>SNAESKIKDCPWYDRGFCKHGPLCRHRHTRRVICVNYLVGFCPEGPSCKFMHPRFELPMGTTEQ[4x];>SNAGSINGVPLLEVDLDSFEDKPWRKPGADLSDYFNYGF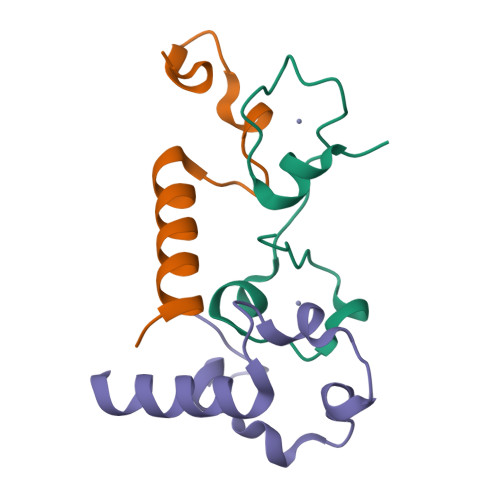NEDTWKAYCEKQKRIRMGLEVIPVTSTTNK[8x]> MNGIHDVGGMDGFGKVM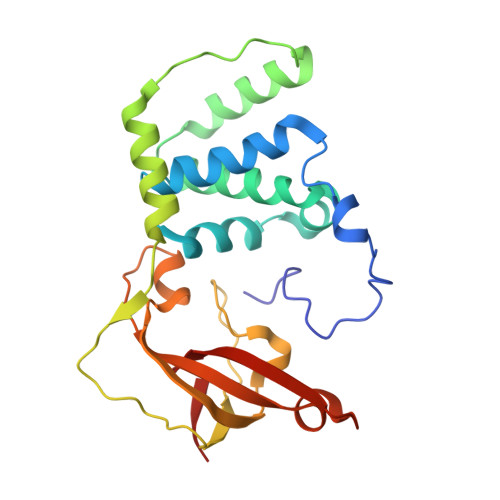YVKEEEDIYFTHDWERLALGLVAGCMAQGLGMKAFDEFRIGIELMRPVDYLTSSYYGHWIATVAYNLVDTGVLDEKELDERTEVFSKKPDTKIPRREDPALVKLVEKALNDGLSPLREISASPRFKVGERIKTKNIHPTGHTRFPRYARDKYGVIDEVYGAHVFPDDAAHRKGENPQYLYRVRFEAEELWGYKQKDSVYIDLWESYMEPVSH>GNSYRHARWWGGAIEEFIQKHGTNFLKDHRFGSYAAIQENALAKWYVNAKGYFEDVANAMEEANEEIFITDWWLSPEIFLKRPVVEGNRWRLDCILKRKAQQGVRIFIMLYKEVELALGINSEYTKRTLMRLHPNIKVMRHPDHVSSTVYLWAHHEKLVIIDQSVAFVGGIDLAYGRWDDNEHRLTDV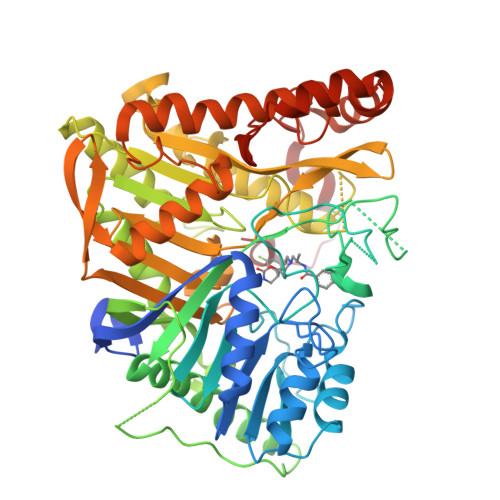GSGSGSGSGSGSGSGSGSGSGSHGETRFWHGKDYCNFVFKDWVQLDKPFADFIDRYSTPRMPWHDIASAVHGKAARDVARHFIQRWNFTKIMKSKYRSLSYPFLLPKSQTTAHELRYQVPGSVHANVQLLRSAADWSAGIKYHEESIHAAYVHVIENSRHYIYIENQFFISCADDKVVFNKIGDAIAQRILKAHRENQKYRVYVVIPLLPGFEGDISTGGGNALQAIMHFNYRTMCRGENSILGQLKAELGNQWINYISFCGLRTHAELEGNLVTELIYVHSKLLIADDNTVIIGSANINDRSMLGKRDSEMAVIVQDTETVPSVMDGKEYQAGRFARGLRLQCFRVVLGYLDDPSEDIQDPVSDKFFKEVWVSTAARNATIYDKVFRCLPNDEVHNLIQLRDFINKPVLAKEDPIRAEEELKKIRGFLVQFPFYFLSEESLLPSVGTKEAIVPMEVWT[6x]> MSGSHHHHHHSGSMSPSPIEEQATRLLKEVPLIDGHNDFPYMIRGWFRNDINGQDAHLYDMPIGQTDLQRLQKGLLGGQFWSAFVPCPKNPDKEVGSLEALRQTLQQLDVIHRLIERHPTILQFADSAASIWSSFRAGRVASLIGIEGLHQIADSVSALR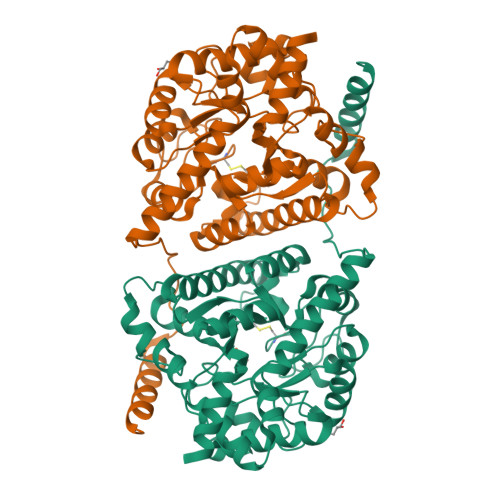MLHRLGVRYVTLTHNCHNAFADAATVSPELHGGLSRKGERLIRELNRMGMMIDLSHTSHEAQTQALRLSRAPVIYSHSSIYSLRAHARNVTDENLHLLHRNRGVVMICFLRELLASEADQATLAHVIDHIIYAGTRIGYEHVGIGSAFDGMLRGPDGLHDVSCYPALVAGLLERGVSEEDVKRVMGLNVIRVLEEVERVAAELQGAGEECLCDELDEVWNEDIKEQLTRERERVRKLGPQK>[2x]MSEQNNAVLPKGVTQGEFNKAVQKFRALLGDDNVLVESDQLVPYNKIMMPVENAAHAPSAAVTATTVEQVQGVVKICNEHKIPIWTISTGRNFGYGSAAPVQRGQVILDLKKMNKIIKIDPEMCYALVEPGVTFGQMYDYIQENNLPVMLSFSAPSAIAGPVGNTMDRGVGYTPYGEHFMMQCGMEVVLANGDVYRTGMGGVPGSNTWQIFKWGYGPTLDGMFTQANYGICTKMGFWLMPKPPVFKPFEVIFEDEADIVEIVDALRPLRMSNTIPNSVVIASTLWEAGSAHLTRAQYTTEPGHTPDSVIKQMQKDTGMGAWNLYAALYGTQEQVDVNWKIVTDVFKKLGKGRIVTQEEAGDTQPFKYRAQLMSGVPNLQEFGLYNWRGGGGSMWFAPVSEARGSECKKQAAMAKRVLHKYGLDYVAEFIVAPRDMHHVIDVLYDRTNPEETKRADACFNELLDEFEKEGYAVYRVNTRFQDRVAQSYGPVKRKLEH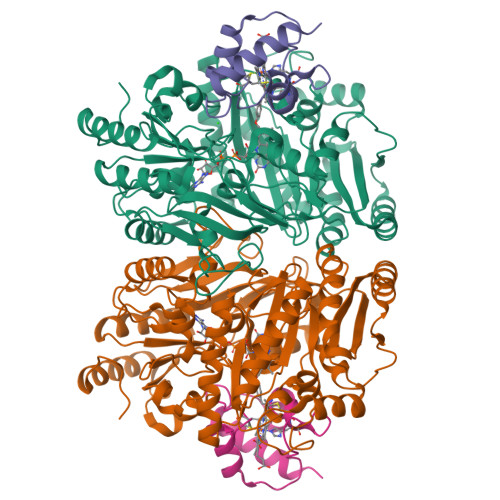AIKRAVDPNNILAPGRSGIDLNNDF;>DSQWGSGKNLYDKVCGHCHKPEVGVGPVLEGRGLPEAYIKDIVRNGFRAMPAFPASYVDDESLTQVAEYLSSLPAPAAQP[2x]>[4x]SFGRDACSEMSIDGLCQCAPIMSEYEIICPANAENPTFRLTIQPKDYVQIMCNLTDTTDYQQLPKKLRIGEVDRVQMRRCMLPGHTPIASILDYLGIVSPTTLIFESDNLGMNITRQHLDRLHGLKRFRFTTRRLTH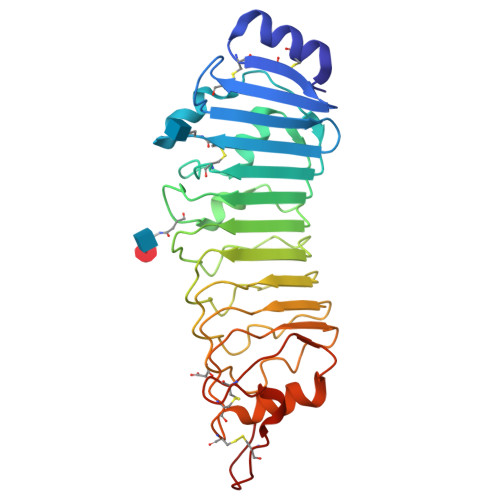IPANLLTDMRNLSHLELRANIEEMPSHLFDDLENLESIEFGSNKLRQMPRGIFGKMPKLKQLNLASNQLKSVPDGIFDRLTSLQKIWLHTNPWDCSCPRIDYLSRWLNKNSQKEQGSAKCSGSGKPVRSIICPTTGENLYFQ>MRILLATDGSPQARGAEALAEWLAYKLSAPLTVLFVVDTRLARIPELLDFGALTVPVPVLRTELERALALRGEAVLERVRQSALAAGVAVEAVLEEGVPHEAILRRARAADLLVLGRSGEAHGDGFGGLGSTADRVLRASPVPVLLAPGEPVELEGALLGYDASESAVRALHALAPLARALGLGVRVVSVHEDPARAEAWALEAEAYLRDHGVEASALVLGGDAADHLLRLQGPGDLLALGAPVRRLVFGSTAERVIRNAQGPVLT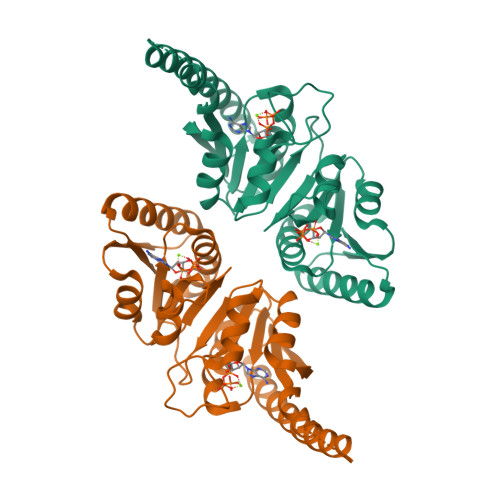AR[2x]A rather recently identified group of PTLBs are the R-type “diffocins” from Clostridium difficile, which constitute the only Gram-positive R-type PTLBs known to date. All R-type PTLBs consist of an inner needle-like rigid tube surrounded by a contractile sheath. Binding triggers extensive conformational changes in the baseplate, accompanied by contraction of the sheath, which, due to extensive interactions, drives the rigid inner tube into the cell envelope. Here, we have determined the crystal structures and SAXS envelopes of the R-type diffocin tube and sheath protein CD1364 and CD1363 in their pre-assembled monomeric state.

The R-type diffocin tube protein CD1364 crystallized in space group P43212 containing one molecule in the asymmetric unit. CD1364 possesses a compact fold with a central β-barrel flanked by two α-helices at both of its open sides. Whereas α-helices α2 and α4 cap the β-barrel on one side, the α-helices at the other protrude away from the β-barrel such that α1 covers the β-barrel of a symmetry-related neighbor. Higher B-factors indicate increased flexibility for α1, which hints at structural changes that may occur during tube assembly. As was suspected from the molecular replacement process, CD1364 shares highest structural and sequence similarity with XkdM from B. subtilis as well as with gp104 from the bacteriophage φ812 tail tube (Nováček et al., 2016), and the overall fold for these proteins is mainly preserved. Notably, in XkdM, α1 does not protrude away from the core of the structure such as in the crystal structure of CD1364 discussed here, but rather caps the β-barrel of the same molecule, again suggesting a high degree of flexibility for this region in both CD1364 and XkdM. Particularly, a prominent loop (K33–G58 in CD1364) is variable and folds into a flexible α-helix in CD1364 (α1), XkdM from B. subtilis and HCP1 from the T6SS of B. pseudomallei, whereas these residues form a protruding β-hairpin in FIIR2 as well as in gp19 from bacteriophage T4 (Zheng et al., 2017). Notably, in the tube protein CD1364, α1, which interacts with a neighboring molecule in the crystal structure, sticks out of the calculated envelope. Comparison reveals that the architecture of the central β-barrel mainly remains unaltered in the assembled tube whereas positions of α-helices α2, α3, and α4 are significantly changed.

> MGPMANMEARNVMSGTWGELWLDGNKVAEVKKFQAKMEFTKEDIIIAGQMGTDTKYMGYKGKGSITLYHVSSRMHKLIGEKIKRGSEPRFVAISKLNDPDSYGAERIAVKNIAFDDLTLADWEVGVKGEIEAPFTFTEYDFLDII>[2x]MDYKDDDDKHHHHHHHHHHENLYFQSYVMGRKLLAEFFGTFWLVFGGCGSAVFAAAFPELGIGFTGVALAFGLTVLTMAYAVGGISGGHFNPAVSVGLTVAGRFPASSLVPYVIAQVAGAIVAAAALYVIATGKAGIDLGGFASNGYGEHSPGGYSLVSALLIEIILTAFFL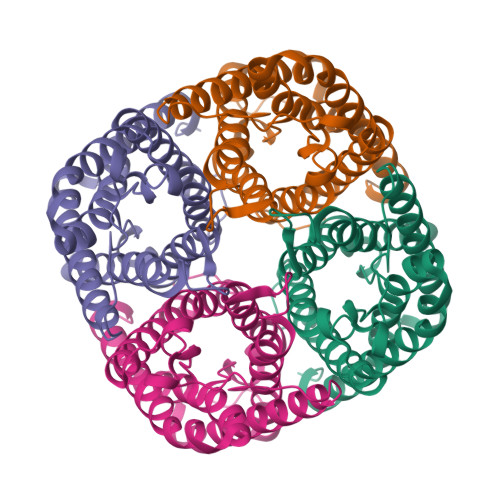IVILGSTHGRVPAGFAPIAIGLALTLIHLISIPVTNTSVNPARSTGQALFVGGWALQQLWLFWLAPIVGGAAGAVIWKLFGEKD[(2~{R},3~{S},4~{S},5~{R})-5-[3-[4-(aminomethyl)-1,2,3-triazol-1-yl]propyl]-3,4-bis(oxidanyl)oxan-2-yl]methyl 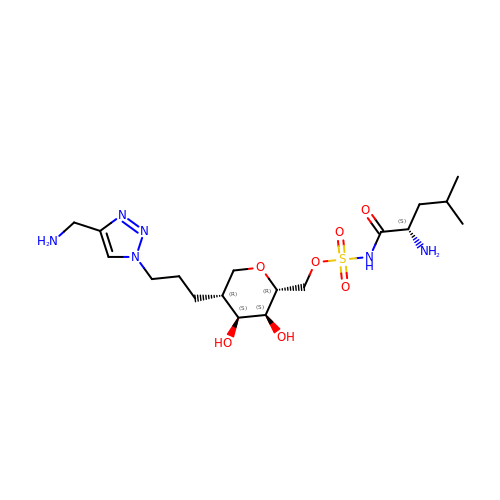~{N}-[(2~{S})-2-azanyl-4-methyl-pentanoyl]sulfamate | C18 H34 N6 O7 S | CBXGRYCGMRFRFP-LMLQULGWSA-N> TQEIYPIKEANGRTRKALIICNTEFKHLSLRYGANFDIIGMKGLLEDLGYDVVVKEELTAEGMESEMKDFAALSEHQTSDSTFLVLMSHGT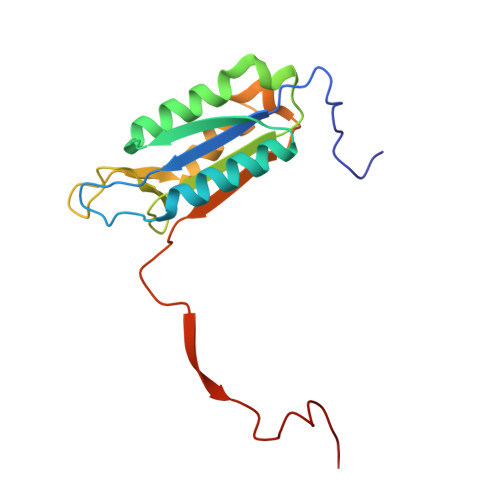LHGICGTMHSEKTPDVLQYDTIYQIFNNCHCPGLRDKPKVIIVQAARGGNSGEMWIRESSKPQLCRGVDL> TETTSFSITKFSPDQQNLIFQGDGYTTKGKLTLTKAVKSTVGRALYSTPIHIWDRDTGNVANFVTSFTFVIDAPSSYNVADGFTFFIAPVDTKPQTGGGYLGVFNSKEYDKTSQTVAVEFDTFYNAAWDPSNKERHIGIDVNSIKSVNTKSWNLQNGERANVV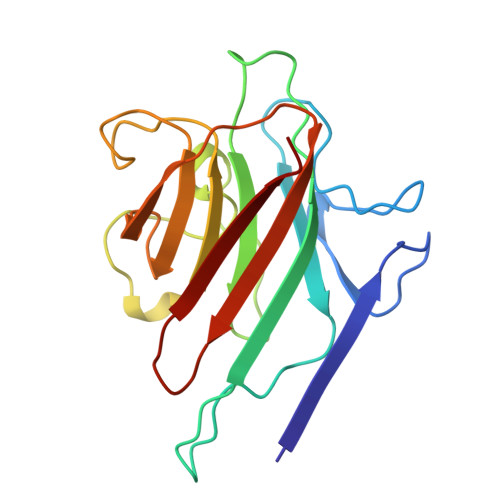IAFNAATNVLTVTLTYPN The major facilitator superfamily (MFS) glucose transporters (GLUTs), encoded by the SLC2 genes, mediate the transmembrane movement of various hexoses and derivatives in different tissues. The two domains, which exhibit a 2-fold pseudosymmetry around an axis that is perpendicular to the membrane plane, enclose a central cavity for substrate accommodation. Exposure of the substrate-binding site to either side of the membrane is achieved through rocker-switch rotation of the two domains as well as local conformational changes exemplified by the bending of TM722. The ligands that specifically bind to the outward- or inward-facing conformers of a transporter, wherein the substrate binding pocket is accessible to the extracellular or intracellular milieu, respectively, are defined as the exofacial or endofacial inhibitors.

Following the same principle for the engineering of XylE-WW, we introduced two Trp substitutions, S64W and I305W, on the extracellular segments of TM2 and TM8 of GLUT3, respectively. This variant will be referred to as GLUT3exo hereafter. The two bulky substituents were expected to trap GLUT3 in an outward-facing conformation. Consistently, the transport activity of GLUT3exo was abolished as measured in proteoliposome-based counterflow assay. To validate the conformational state of GLUT3exo, we resolved the crystal structure of GLUT3exo in complex with glucose at 2.1 Å using LCP crystallization approach. As expected, GLUT3exo exhibits an outward-facing state with a glucose molecule standing in its central pocket. The two bulky residues, Trp64 and Trp305, wedge into the two lateral interfaces of the N and C domains, i.e., between TM2 and TM11 and between TM5 and TM8, respectively, to lock the outward-facing conformation. Except for these two Trp substitutions, the structure of GLUT3exo is nearly identical to that of the outward-occluded GLUT3-glucose with a root-mean-square deviation (RMSD) of 0.236 Å over 402 Cα atoms. Consistent with its trapped outward-facing conformation, GLUT3exo can only recognize the exofacial inhibitor phloretin, with a KD of 15.5 ± 1.5 μM. Its affinity with the endofacial inhibitor CCB was not detectable.

> MHHHHHHHHHHSGDEVDAGSGQVDAGTMGTQKVTPALIFAITVATIGSFQFGYNTGVINAPEKIIKEFITKTLTDKGNAPPSEVLLTSLWWLSVAIFSVGGMIGSFSVGLFVNRFGRRNSMLIVNLLAVTGGCFMGLCKVAKSVEMLILGRLVIGLFCGLCTGFVPMYIGEISPTALRGAFGTLNQLGIVVGILVAQIFGLEFILGSEELWPLLLGFTILPAILQSAALPFCPESPRFLLINRKEEENAKQILQRLWGTQDVSQDIQEMKDESARMSQEKQVTVLELFRVSSYRQPIIISIVLQLSQQLSGINAVFYYSTGIFKDAGVQEPWYATIGAGVVNTIFTVVSLFLVERAGRRTLHMIGLGGMAFCSTLMTVSLLLKDNYNGMSFVCIGAILVFVAFFEIGPGPIPWFIVAELFSQGPRPAAMAVAGCSNWTSNFLVGLLFPSAAHYLGAYVFIIFTGFLITFLAFTFFKVPETRGRTFEDITRAFEGQAHGADRSGKDGVMEMNSIEPAKETTTNV> MANKAVNDFILAMNYDKKKLLTHQGESIENRFIKEGNQLPDEFVVIERKKRSLSTNTSDISVTATNDSRLYPGALLVVDETLLENNPTLLAVDRAPMTYSIDLPGLASSDSFLQVEDPSNSSVRGAVNDLLAKWHQDYGQVNNVPARMQYEKITAHSMEQLKVKFGSDFEKTGNSLDIDFNSVHSGEKQIQIVNFKQIYYTVSVDAVKNPGDVFQDTVTVEDLKQRGISAERPLVYISSVAYGRQVYLKLETTSKSDEVEAAFEALIKGVKVAPQTEWKQILDNTEVKAVILGGDPSSGARVVTGKVDMVEDLIQEGSRFTADHPGLPISYTTSFLRDNVVATFQNSTDYVETKVTAYRNGDLLLDHSGAYVAQYYITWDELSYNHQGKEVLTPKAWDRNGQDLTAHFTTSIPLKGNVRNLSVKIREATGLAWEWWRTVYEKTDLPLVRKRTISIWGTTLYPQVEDKVEND

The cholesterol-dependent cytolysin (CDC), pneumolysin is a virulence factor of the human pathogen Streptococcus pneumoniae (pneumococcus)2, the leading cause of bacterial pneumonia and a major agent of meningitis and septicaemia as well as debilitating diseases such as otitis media, septic arthritis, keratitis and sinusitis. A central feature of the toxin is the formation of transmembrane pores in cholesterol-containing membranes, which lyse or disrupt cell functioning, depending on the concentration. Pneumolysin and other CDCs bind to mammalian membranes through a tryptophan-rich loop and a threonine-leucine pair within a membrane-binding domain at the base of the toxin. Once bound to the membrane, monomers then oligomerise to form a pre-pore complex that subsequently undergoes a complex set of structural transitions to form a transmembrane pore, typically comprising 30–50 subunits.

In this work, we have determined the structure of pneumolysin at 1.98 Å resolution. The best crystals were obtained from protein containing substitutions Asp385Asn and Cys432Ala. The asymmetric unit contained a single molecule having the characteristic four domain structure of a CDC, with three non-contiguous domains (domains 1–3) linked to the C-terminal membrane-binding domain via the strap-like domain 2. The tryptophan-rich loop, projects from the base of domain 4 in the structure of full-length pneumolysin, reflecting the likely membrane-binding conformation. Notably, two of the tryptophan residues, Trp433 and Trp435, shown previously to be important for membrane binding and cell lysis, project outwards, so are in position to allow interactions with a lipid bilayer. In the structure of full-length pneumolysin, domain 4 is offset by ~30° relative to the plane of the long axis of domains 1–3, such that the toxin resembles a bend rod from the side. A striking feature of pneumolysin crystals, is that monomers pack side-by-side in the crystal lattice, resembling the molecular packing of the pre-pore complex. The interface between pneumolysin molecules is created by the concave face of one monomer packing against the convex face of its neighbour. Intermolecular contacts are made by all four domains, but mostly involve domains 1 and 4. Although most of the residues at the interface are polar, there are relatively few polar intermolecular interactions: salt bridges between Asp8 and Arg226 and Glu434 and Arg399 and hydrogen bonds between the side-chain of Asn339 and the carbonyl group of Pro87, and between the hydroxyl group of Tyr461 and the amine and carbonyl groups of His407.>MKPHALIGLLAGMLLSSSLYAADSTKPLPLHIGGRVLVESPANQPVSYTYSWPAVYFETAFKGQSLTLKFDDDQNIFRLIVDDKAPVVINKPGKVDYPVESLAPGKHRVRLEKLTETQSTSGRFLGFYTDPSAKPLALPKRKRQIEFIGDSFTVGYGNTSPSRECTDEELFKTTNSQMAFGPLTAKAFDADYQINASSGFGIVRNYNGTSPDKSLLSLYPYTLNNPDQLYHNKHWKPQVIVIGLGTNDFSTALNDNERWKTREALHADYVANYVKFVKQLHSNNARAQFILMNSDQSNGEIAEQVGKVVAQLKGGGLHQVEQIV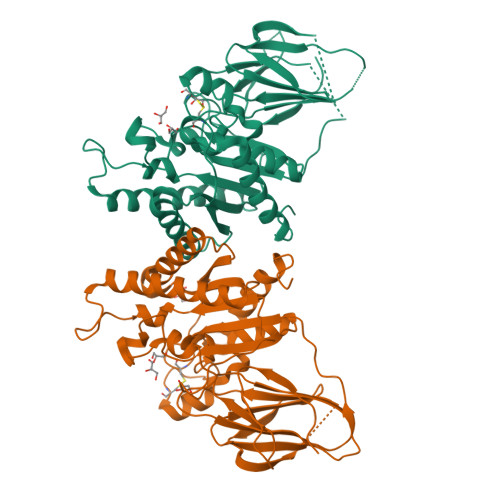FKGLDYSGCHWHPSANDDQLLANLLITHLQQKKGIWLEHHHH[2x]>[2x]MSNVPHKSSLPEGIRPGTVLRIRGLVPPNASRFHVNLLCGEEQGSDAALHFNPRLDTSEVVFNSKEQGSWGREERGPGVPFQRGQPFEVLIIASDDGFKAVVGDAQYHHFRHRLPLARVRLVEVGGDVQLDSVRIF

Galectins (Gals) are a family of animal lectins that bind β-galactose-containing glycoconjugates, and their carbohydrate recognition domain (CRD) has a conservative amino acid sequence. To date, 16 mammalian galectins have been discovered, and galectin-7 (Gal-7; also termed p53-induced gene 1 product), belonging to prototype galectins, is a multifunctional effector by productive pairing with distinct glycoconjugates and protein counter-receptors in the cytoplasm and nucleus, as well as on the cell surface. Gal-7 participates in diverse processes, such as controlling apoptosis, cell migration and cell adhesion. Gal-7 was crystallized in complex with glycerol under two different conditions.

The two refined structures, structure 1 (homodimeric Gal-7 binds two glycerol molecules) and structure 2 (homodimeric Gal-7 binds three glycerol molecules), were crystallized using two different conditions, one at a relatively low concentration of PEG3350 (12%) and the other at a higher concentration (20%). As with all other galectins, structures 1 and 2 adopt the typical “jelly-roll” fold formed by sandwiching two anti-parallel β-sheets that consist of six (S1-S5) and five (F1–F5) β-strands and a short α-helix connecting strands S2 and F5 at 1.8 Å and 2.0 Å resolution, respectively. Our Gal-7 in complex glycerols as dimers in the P212121 space group is the same as previously reported for Gal-7. The positions of residues His 50, Asn 52, Arg 54, Val 61, Asn 63, Trp 70 and Glu 73 coordinate with glycerol. In our crystal structure, the C and O atoms of glycerol occupy similar positions as the C4, C5, C6 and O4, O5, and O6 atoms of galactose in the lactose-bound structure. It indicates that glycerol is a small ligand of Gal-7. Discrepancies between structure 1 and structure 2 in monomer A are due to the absence or presence of GOL C. B-factors of structure 1 suggests that the N-terminal regions are very flexible, while the N-terminal region of structure 2 is relatively stable due to the binding of GOL C. Just like Gal-7 structure 1 in the crystallization condition (20% PEG 3350, 0.2M magnesium chloride, 0.1M HEPES, pH7.5), no electron density of glycerol was found in GOL C sites, but glycerol electron density was found in GOL C sites in structure 2 of Gal-7 under another crystallization condition (0.1M HEPES, pH7.5, 12% PEG 3350).>GHMSTFLPAPLQCGRFELTFERPLVMGILNATPDSFSDGGRFLARDDALRRAERMIAEGADLLDIGGESTRPGAPPVPLDEELARVIPLVEALRPLNVPLSIDTYKPAVMRAALAAGADLINDIWGFRQPGAIDAVRDGNSGLCAMHMLGEPQTMQVGEPDYGDVVTDVRDFLAARAQALRDAGVAAERICVDPGFGFGKAVVDDNYALLAALPDTAPARPDGRAYPILAGMSRKSMLGAVIGGKPPLERVAASVAAALCAVERGAAIVRVHDVAATVDALSVWNAVRAA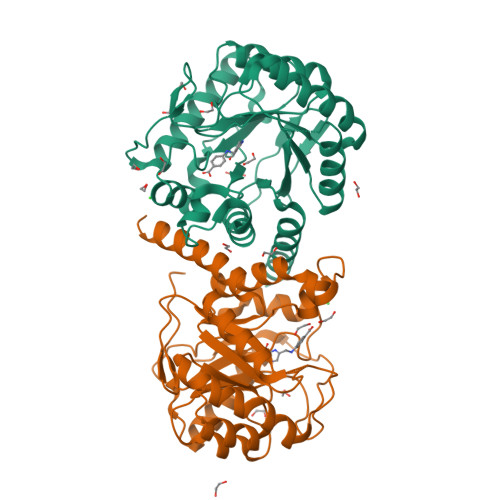ARQR[2x]>MSLIYEDLVKSLDSKQQAYVDLKLPDPTNGEFLLAVFHMIPGGDLNVLQAAAEIAAESSTGTNIKVSTETAFSRTMNARVYQLDLERELVWIAYPWRLFDRGGNVQNILTYIIGNILGMKEIQALKLMDIWFPPSMLEQYDGPSYTVDDMRKYLDVYDRPILGTIVKPKMGLTSAEYAEVCYDFWVGGGDFVKNDEPQANQDFCPYEKMVAHVKEAMDKAVKETGQKKVHSFNVSAADFDTMIERCEMITNAGFEPGSYAFLIDGITAGWMAVQTLRRRYPDVFLHFHRAAH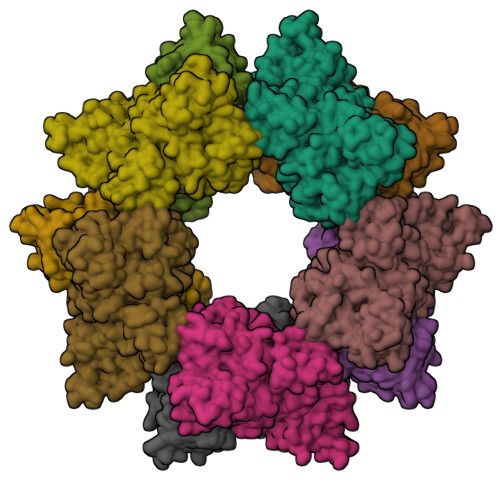GAFTRQENPIGFSVLVLSKFARLAGASGIHTGTAGIGKMKGTPAEDVVAAHSIQYLKSPGHFFEQTWSKIMDTDKDVINLVNEDLAHHVILEDDSWRAMKKCCPIVSGGLNPVKLKPFIDVMENVDFITTMGSGVHSHPGGTQSGAKALVQACDAYLQGMDIEEYAKDHKELAEAIEFYLNR[5x]> MKIGIIGAGQLARMLSLAGTPLGLEFHCLGKNGDCAEEVVKTVTDIELTKVNDVVAWAKQFDVITFENENISHELIKAINHEVSVYPSAKAIAISQDRLLEKSFMQDHGIATAKFVNIDSLAKLQSAVDDHGLPAILKTRRFGYDGKGQFVIRSQEDITKAWDVLKDAPDGLIYEAFVDFDYEVSQICTADLKGNIAFYPLARNTHKQGIIVESEAPFENVVLAEKAQQIAKILVKEFAYVGTLAIEFFVKGDELIV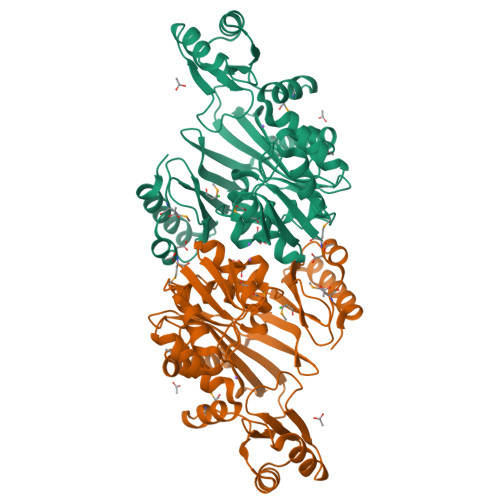NEIAPRVHNSGHWSIDGAVTSQFENHVRAIAGLILGDTTSRKTVMLNCIGGMPATKDLAALDRVKIHSYNKEPRKGRKVGHLNLNLNDETDEYQLLQVKKLIALSEEIAGNLYFQ> MKDLLNLFNQQRQTLDFDAIKIALASPDLIRSWSYGEVKKPETINYRTFKPERDGLFCAAIFGPIKDYECLCGKYKRMKHRGVVCEKCGTEVTLAKVRRERMGHIDLASPVAHIWFLKSLPSRIGLMLDMTLRDIERVLYFEAYVVTEPGLTPLERRQLLTEEQYLTARQEYNDDFDAAMGAEAVYELLRTIDLQSEMTRLREEIASTGSETKLKRLTKRIKLIEAFLESGNRPEWMVMTVLPVLPPDLRPLVPLDGGRFATSDLNDLYRRVINRNNRLRRLLELNAPDIIVRNEKRMLQESVDALLDNGRRGRAITGTNKRPLKSLADMIKGKQGRFRQNLLGKRVDYSGRSVITVGPYLKLHQCGLPKKMALELFKPFVFAKLQRRGLATTIKAAKKLVEREEAEVWDILEEVIREHPVLLNRAPTLHRLGIQAFEPVLIEGKAIQLHPLVCTAFNADFDGDQMAVHVPLSLEAQLEARALMMSTNNILSPANGEPIIVPSQDVVLGLYYMSRALENKKGEGMVFANTSEVKRAYDNRVVELHAKVKVRITQVDVDAVDGKRTSGTSIVDTTVGRALLSEILPEGLPFQLANTEMTKKNISRLINSSYRLLGLKDTVVFADKLMYTGYAYATRAGVSIGIDDMLIPDEKKGILTEAEAEVLEIQEQYQSGLVTAGERYNKVVDIWSRTSERIAKAMMDTIGTEKVENAKGETIDQKSMNSLYIMADSGARGSQAQIRQLAGMRGLMARPDGSIIETPIKANFREGLNVQEYFNSTHGARKGLADTALKTANSGYLTRRLVDVAQDVVITEIDCGTTEGLIMTPIVEGGDVVEPLKERVLGRVVAEDVYLPGNDEEPIVTRNTLLDEAWVAKLEDASVQSVKVRSTISCESSFGVCARCYGRDLARGHQVNIGEAVGVIAAQSIGEPGTQLTMRTFHIGGAASRAAAVDNITVKTTGSVKFNNLKS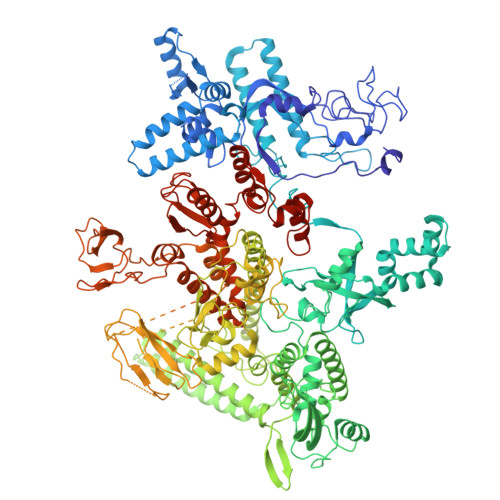VAHASGSLVAVSRSGELSVLDGHGRERERYKLPYGATITAKDGDAVKAGQSVANWDPHNHPIVSEVAGFIRFIDFVDGVTVIEKTDELTGLASREITDPKRRGAHAKELRPIVRIVDGKGNDLTIPNTDLPAQYLLPPRSIVNLQDGAAVGVGDVVAKIPQEASKTRDITGGLPRVADLFEARKPKDPAILAERSGIISFGKDTKGKQRLIIKDTDGSEHEELIPKYRQIIVFEGEHVTKGETVVDGEPSPQDILRLLGVEPLAAYLVKEIQDVYRLQGVKINDKHIEVITRQMLRKVEIVDQGNSKFLNGEQVERQRVIEENARLVKRNELPAKYDPVLLGITKASLATESFISAASFQETTRVLTEAAVRGTRDNLRGLKENVIVGRLIPAGTGLAYHAGRRKASGLTDSEMETLSGKPAGAEPVAALADAGADEE In this study, two fungal chimeric class I TrTSs, Talaromyces verruculosus talaropentaene synthase (TvTS) and Macrophomina phaseolina macrophomene synthase (MpMS), were characterized. Both enzymes use dimethylallyl diphosphate and isopentenyl diphosphate or hexaprenyl diphosphate as substrates, representing the first examples, to our knowledge, of non-squalene-dependent triterpene biosynthesis. Structural analyses of the terpene cyclase domain of TvTS and full-length MpMS provide detailed insights into their catalytic mechanisms. In summary, a novel family of chimeric class I TrTSs converting HexPP into triterpenes was identified for which two subclasses can be distinguished.

Because recombinant full-length TvTS was insoluble, for in vitro assays the TvTS-PT and TvTS-TC domains were expressed individually. The structural basis of the cyclization mechanism was investigated by determination of the crystal structure of apo TvTS-TC by soaking with the non-reactive substrate surrogate 2,3-dihydro-HexPP. Although 2,3-dihydro-HexPP was not clearly observed and we cannot completely exclude the possibility that the observed electron density originated from polyethylene glycol (PEG) used in the crystallization buffer, the disordered regions in the apo structure, especially the DDXXD motif and the active site loop D173–D182, appeared clearly structured following soaking with the substrate surrogate. This observation suggests that a major conformational change occurs in TvTS following substrate binding that facilitates active site closure. The TvTS active site contains the conserved DDXXD and NSE motifs and other residues that interact with the substrate’s diphosphate. Aromatic residues in TvTS-TC (F65, F89, F187, W188 and W310) are observed in positions analogous to those in PaFS (F65, F89, F196, W197 and W319), while the PaFS residues at the bottom of the active site (M221, W225, M309, S312 and N316) are substituted with smaller residues in TvTS (A212, Y216, G300, G303 and S307). These differences create a larger pocket in TvTS-TC that is composed of a tunnel to accommodate two additional (non-reacting) isoprene units of HexPP, sticking out from a ball-shaped cavity in which the four reacting isoprene units are located. The high similarity between the AlphaFold2-predicted model and the crystal structure of TvTS-TC offers a basis for the discovery of additional chimeric fungal TrTSs through structural prediction, which is not possible from amino acid sequence analyses.

> MDFKYSRELKLESLDALNLTEGIPLRVNENIDLEFRGIERAHSDWERYVGKLNGFHGGRGPQFGFVSACIPECLPERMETVSYANEFAFLHDDMTDAASKDQVNGLNDDLLGGLDFTTEARSSASGKQQMQAKLLLEMLSIDRERTMVTIKAWADFMRGAAGRDHHRGFSSLDEYIPYRCADCGEKFWFGLVTFAMALSIPEQELELVQRLAQNAYLAAGLTNDLYSYEKEQLVAERSGTGQVFNAIAVIMQEHSVSISEAEDICRGRIREYAAKYVRDVADLRAKNELSRDSLAYLETGLYGISGSTAWNLDCPRYQVSTFVDFKTP> MEKFVLSLDEGTTSARAIIFDRESNIHGIGQYEFPQHYPRPGWVEHNPEEIWDAQLRAIKDAIQSARIEPNQIAAIGVTNQRETTLVWDK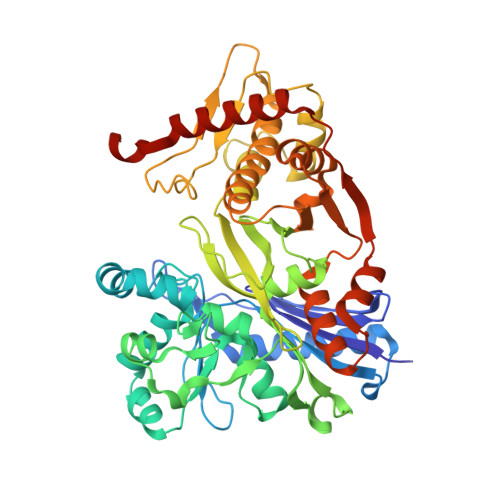DGKPLYNAIVWQCRRTAEMVEEIKREYGTMIKEKTGLVPDAYFSASKLKWLLDNVPGLREKAEKGEVMFGTVDTFLIYRLTGEHVTDYSNASRTMLFNIKKLDWDDELLELFDIPESVLPEVRESSEVYGYTKKELLGAEIPVSGDAGDQQAALFGQAAFEAGMVKATYGTGSFILVNTDEMVLYSDNLLTTIAWGLNGRVSYALEGSIFVTGAAVQWLRDGIKIIKHASETEELATKLESNEGVYFVPAFVGLGAPYWDQFARGIIIGITRGTGREHLARATLEAIAYLTRDVVDEMEKLVQIKELRVDGGATANDFLMQFQADILNRKVIRPVVKETTALGAAYLAGLAVDYWADTREIAELWKAERIFEPKMDEKTRERLYKGWKEAVKRAMGWAKVVDSAKSN>[2x]MASGMTVTDAGADQPIVFVNRAFSTITGYAPNEVLGRNARFLQGPQTDAATVARLREAIAAARPIQERILNYRKDGQPFWNQLSISPVRDETGNVVAFVGVKTDVTAHHHHHH

Flavin-binding fluorescent proteins (FbFPs), engineered from prokaryotic and eukaryotic light, oxygen, voltage (LOV) photoreceptors, are promising fluorescent reporter proteins. Their small size (about 10 kDa for monomeric FbFPs such as the improved LOV (iLOV) protein derived from Arabidopsis thaliana phototropin photoreceptors) and their oxygen-independent fluorescence make them ideal reporters to monitor transport and anaerobic biological processes. In contrast to GFP-like fluorescent reporter proteins, whose absorption and fluorescence maxima can be tuned by exchanging certain chromophore-constituting amino acids, the absorption and fluorescence of FbFPs and other flavoproteins depends on noncovalently bound flavins, whose structure cannot be influenced by mutation. Using spectroscopy, X-ray crystallography, and quantum mechanics molecular mechanics calculations, we provide a firm structural and functional understanding of spectral tuning in FbFPs.

To verify the transferability of the mutation, we introduced the corresponding I52T mutation into CagFbFP–Q148K. The resulting purified protein showed very similar spectral properties as iLOV–V392T–Q489K, that is, basically no shift in the absorption maximum relative to parental CagFbFP (compare solid red line and gray dashed line) and a 7-nm red-shifted fluorescence-emission maximum (compare gray dashed line and solid red line). We readily obtained orthorhombic crystals for CagFbFP–I52T–Q148K (space group P21212, two molecules per asymmetric units) that diffracted up to 1.8 Å. Compared with the blue-shifted iLOV–Q489K and CagFbFP–Q148K variants, the red-shifted double variant shows a closed FMN binding pocket with no unlatched C terminus (C-α atom core RMSD: 0.48 Å with 102 aligned residues). The introduced threonine (T52) shows two conformations in both subunits, one with the side-chain oxygen facing toward G146 and a second one with the side-chain oxygen facing toward F69 (approximate occupancies of the two conformations are 65% and 35%, respectively). K489 adopts one major conformation in both subunits (approximate occupancy 65%) in which the side chain extends toward the introduced T52 and the FMN moiety. Interactions between both threonine conformations and the lysine are feasible with interatomic distances between the lysine NZ atom and the threonine side-chain oxygen of 2.5 Å or 2.6 Å in both subunits. It is remarkable that the double mutation (CagFbFP–I52T–Q148K) forces the lysine into a new conformation by hydrogen bonding with threonine, thus preventing the bending of the C terminus, which restores a nearly “native” closed LOV-core conformation.>MRKFILSLSILLSALLVACSSRNHYGDTGSLAGLQAMADSKYTRAQKKQKMGKIREMALKETALSVGAQAGLAWRAKIIDEQLNKQARNLDAIYDFNSLVLEHNILPPVLLEGRNTLNLADAQSIRISDRTYKVAKQAHFITTPPTWRQYLWMDYVKPEAPNVTLLPKTKAEKEIWCIYTERGWKNGIDQANTILEENIARIKEDFGGMILYRKLLAMNMVSPPYVSHTDLGVTGDGSEIHIDDRVLRITALPELNVNSAEWRAAVAKDENALERFKNMEKLANQAKIVITNKSWQPIIAPVS[13x];>[26x]MNNNKIVIMFIFSALLAGCAGTMKFKKPPINNPSDDATIKLAEAAVSVSDSMLEMAKVEKVITPPSKDNTLTIPNAYNLQARASVDWSGPIEELTARIAKAAHFRFRVLGKSPSVPVLISISTKDESLAEILRDIDYQAGKKASIHVYPNSQVVELRYAKIYS;>[13x]MMKKYDQLCKYCLVIGLTFSMSCSIYAADQSDDAQQALQQLRMLQQKLSQNPSPDAQSGAGDGGDNAASDSTQQPNQSGQANAPAANQTATAGGDGQIISQDDAEVIDKKAFKDMTRNLYPLNPEQVVKLKQIYETSEYAKAATPGTPPKPTATSQFVNLSPGSTPPVIRLSQGFVSSLVFLDSTGAPWPIAAYDLGDPSSFNIQWDKTSNTLMIQATKLYNYGNLAVRLRGLNTPVMLTLIPGQKAVDYRVDLRVQGYGPNAKSMPTEEGIPPSANDLLLHVLEGVPPPGSRRLVVSGGDARAWLSNEKMYVRTNLTILSPGWLASMTSADGTHAYEMQKSPVLLVSWHGKVMQLKVEGL;>MRSLRTNYIYVLFKTTGLLFLLLLSACNRSGYIPENEVPKLPCRVDGACDATIIKMMTDLNKKGIKVASVGQNYLISIPASALFADQSPRLNWASYSLLNEIAAFLKQFRKIAITVTSYSSKYVSVKRERALTLARSRVVSEYLWSQGVDSRIIFTQGLGSDKPITSYTLGGDRSPNARVEITFRRAVA[13x];>[52x]AAAAAAAAAAAAAAAAAAAAAAAAAAAAAAAAAAAAAAAAAAAAAAAAAAAAAAAAAAAAAAAAAAAAAAAAAAAAAAAAAAAAAAAAAAAAAAAAAAAAAAAAAAAAAAAAAAAAAAAAAAAAAAAAAAAAAAAAAAAAAAAAAAAAAAAAAAAAAAAAAAAAAAAAAAAAAAAAAAAAAAAAAAAAAAAAAAAAAAAAAAAAAAAAAAAAAAAAAAAAAAAAAAAAAAAAAAAAAAAAAAAAAAAAAAAAAAAAAAAAAAAAAAAAAAAAAAAAAAAAAAAAAAAAAAAAAAAAAAAAAAAAAAAAAAAAAAAAAAAAAAAAAAAAAAMRNLMRCLIMIKSLIKGVDMSRKLAKTRILGYGLMICFLAGCFHPPYNNFQPDRRAVKRVGVDTGIGAVAGAIASGTASGTLIGAAAGGTVGLVASIYRDSKRKIIRDLQKQDIQYVEYGDTRTLIIPTDKYFMFSSPRLNEICYPGLNNVIRLLNFYPQSTIYVAGFTDNVGSRSHKRKLSQAQAETMMTFLWANGIAAKRLKAEGYGDKNAISDNAIIHGSAQNRRIEIQWFTSPAQPPQPQMAYVK

The Type IV Secretion System (T4SS) is a potent weapon used by some bacteria to infect their host and can deliver effector proteins into eukaryotic cells as well as DNA and/or toxins into bacterial neighbors. In the Gram-negative pathogen L. pneumophila, the Dot/Icm T4SS delivers ~300 effector proteins to the cytoplasm of host cells, in some cases causing Legionnaires’ Disease. Central to assembly of the apparatus are five proteins that define the core complex: DotC, DotD, DotF, DotG, and DotH. The map can be divided into two major regions: an outer membrane cap (OMC) and a hollow periplasmic ring (PR).

Using symmetry and focused refinement, we determined a 3.5 Å resolution map of the OMC disk and a 3.7 Å map of the PR. The OMC disk makes up the pinwheel-shaped portion of the T4SS and is organized into a thick central region with 13 arms extending radially outward. The disk is also thin compared to other structurally characterized T4SS OMCs and contains no distinct inner or outer layers. Within the disk, we unambiguously traced and identified DotC, DotD, DotK and DotH along with the protein Lpg0657 (Goodwin et al., 2016; Figure 2B, Figure 2—figure supplements 1 and 2). Notably, rather than an equimolar ratio, the components of the OMC exist at a ratio of 2:1:1:1:1 (DotD:DotC:DotH:DotK:Lpg0657). At the center of the OMC is an elongated fold that is comprised of α-helices and β-strands that we have identified as DotC (residues 58–161 and 173–268). On the peripheral side, DotC makes contact with two copies of DotD, which we have called DotD1 and DotD2. DotK contacts the C-terminal domain of DotD2, whereas Lpg0657 interacts with the N-terminal α-helices of both DotD1 and DotD2. On the periplasmic side of the OMC is another small globular fold that we identified as the C-terminal domain of DotH. Within the OMC disk we traced three poly-alanine chains that could not be unambiguously identified as any component of the Dot/Icm T4SS.>[4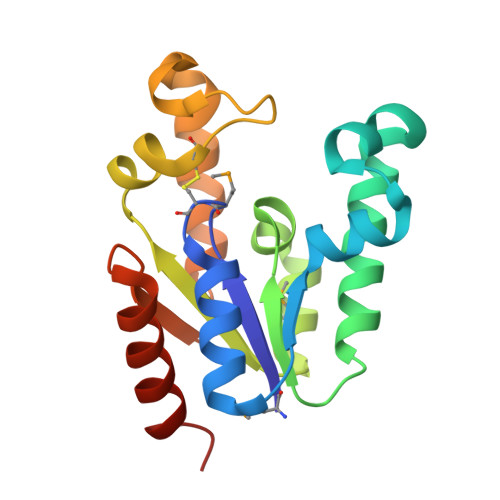x]MRIYLIGFMCSGKSTVGSLLSRSLNIPFYDVDEEVQKREGLSIPQIFEKKGEAYFRKLEFEVLKDLSEKENVVISTGGGLGANEEALNFMKSRGTTVFIDIPFEVFLERCKDSKERPLLKRPLDEIKNLFEERRKIYSKADIKVKGEKPPEEVVKEILLSLEGNALGG> MHHHHHHMYDATRINQDLFVGGFYGDVIAMRHFVRQNNV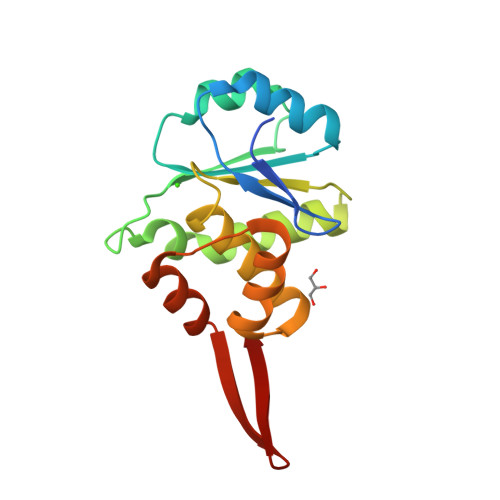GCVVSLIDSDVAPIKRALYLPDGDHLHVHCEDDAKCGALADNLEMLFNYLWLKIHNEHKTVLIHCHAGVSRSATLAIYYIMRTNQIDYEQAFQYVYGKRAVHPSEHFVELLKGKCVYSYVDNKLVVRVE> MENLGDKLSISQVYHLAQEYRDHAYSIANKIGSEEGLKQYYGLMNMSIQMFQLLKTKCTLSVLEDSKVTFEMVELLIQETYNFDLAELYISSLKERLQTHQSDTDLVEEIMRCEFLLLHDLPLMRDSKFHYKIALRNCNELVQYMVNLQDELYQNWASVFQYVGVMLCI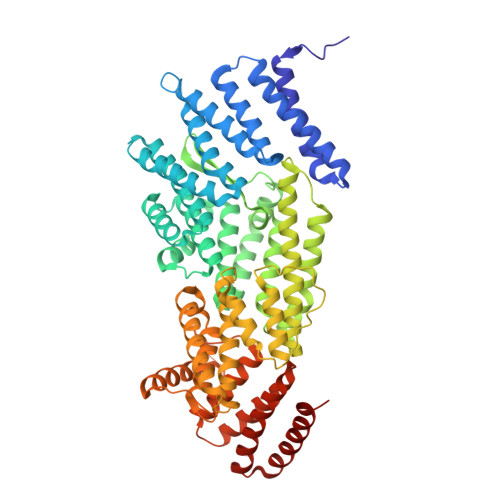KLKQHRRVKTSFHGLLSQCREKSQWKWFLNLCYVNYLLNERFPIPEDALQELRSTELHTVGPELYAWKLALEMVIQLCKDGNITDHLNEFKNFFDTNKQSLVTNEGKGCVIKIMPRIALKVELPMIFHYKELKNILLLLQSVSYIVNCYDEKGNFSRKFLPKVYSTTQKLIKNIAAGGVSMNELDSRIQTYKSILEFCEFYKVWEQTLLKGAVVTTESPKLGPSPGYVRLLQAMKVQFEGGGAVEEYTRLAQSGGTSSEVKMISLLNCYTVQAARVSRCSGDKQGELVEQCNKVWLQVEKLLQETDLQFNPIWECTVTILWLFSHFEPFSWNPLPCSDKQRAEYVSKLREFYSSNKFVAGEAVADNRFKLKKALLLQILVNYLGGRMLEHDLGEIYAISAKCFDMCRQQGGMRKVQYVIGIWHLMNCTVAMRGKDVALTNAKLEALVKQITSVKQ> SMAKRVFFSFHYQDVIDFRVNVVRNHWVTKLNQSAAGVFDASLWEDAKKTSDIALKRLINGGLNNTSVTCVLIGSQTFNRRWVRYEIMKSIEKGNKIIGIHINAFKDKYGNIKSKGPNPFDYLGYQYSSDGKQLHLYEWTGGKWEEYKDLAP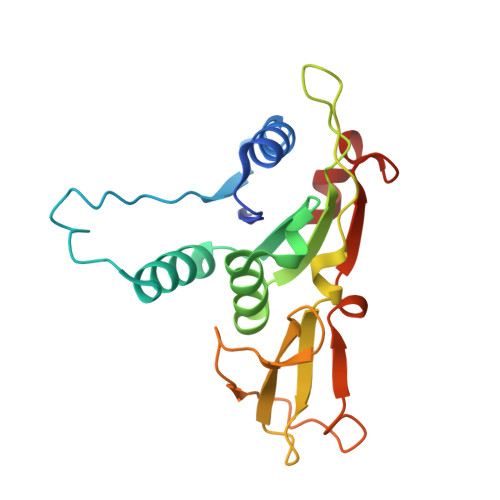YRVNQIAPESLRGKFYSLSSVYRVYDWVADDGYNKFSSWVN>MSEQITGSTPRIYYRGTKDSSVTRSTGSTTTLPLHRPLIMFFGQKGPTVPTWIDPVKFEDIYGSETTNLSGVYCTHSTPFIKEAIAAGNQFMALRLEPSDIPDVATLGLSVDWVKTKIDDYERNDDGTYKLDTNGDKIPLATQIDGIKFRFVLEKIETNESGVSQYKKRTAKAGTIGTEATPSTITPLADFRCRFKSSLGANTALRIWAPTINSAQAADADLQARIKSFLYRFQILTRADKASSPTIFETIYNEPSLSVGFGENLVDPQTEVVYD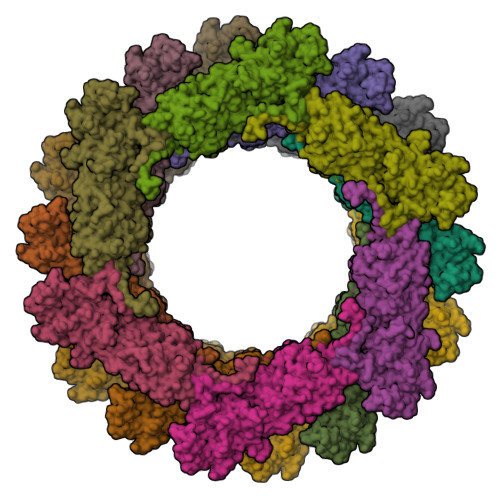FVERIDSRYNDEDPSTYLMSPLDTPYLYQANIDSVLTAIQELEAPFDTVSADEDDLYQINLFGAQTVEGVPYHAVQILGVLDGGVTLTETATNYLQGGGDGTLGNDSFNAAAYAVLSNLSNNAAFNITNYARYPFNAFWDSGFDLKTKQTIPQLIGLRADTWIALSTQDISSDFNSNEEEESIALSLMSRVSAFPDSSDFGTPAFRGMIVGGAGYYTETTRKLPVPLTLDRFRAYCRYAGASDGVLKPEYAVDEGDARKVQVVKSINNLDKSWRVRRAQWNNNLVYVEDYDTNSQFYPGQQSFYSEQGSVLKAAIVGLCVANLNRFAFEAWRDLTGTQKLTDDQLIERSDDAVSTRGTGAFDDRLIFTPHSEITQADKERGYSWSMRIDFGANAFRTVMDMSSVAYTREELANG[18x]>[2x]VAFTEKQDALVSSSFEAFKANIPQYSVVFYTSILEKAPAAKDLFSFLANGVDPTNPKLTGHAEKLFALVRDSAGQLKASG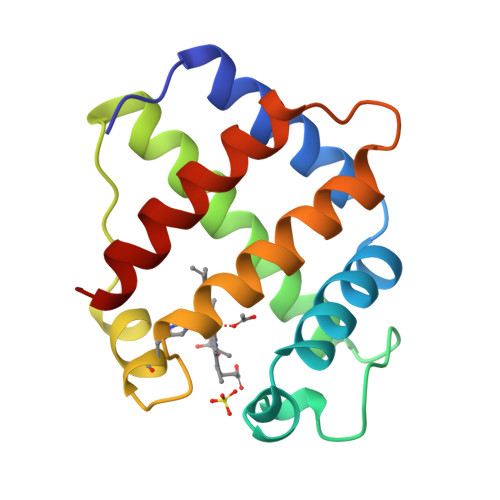TVVADAALGSVHAQKAVTDPQFVVVKEALLKTIKAAVGDKWSDELSRAWEVAYDELAAAIKKA N-(3-hydroxy-9,10-dioxo-9,10-dihydroanthracene-2-sulfonyl)glycine | C16 H11 N O7 S 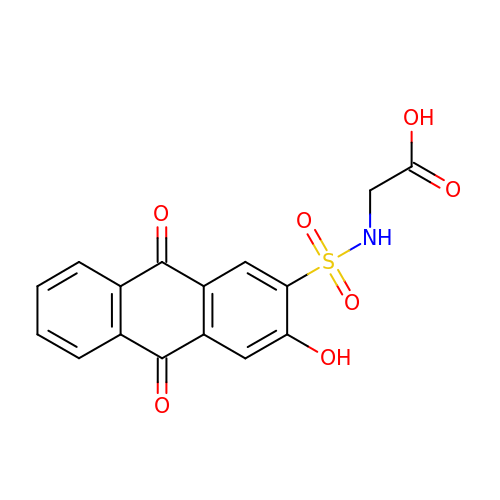| YKNJQQVUXNATBD-UHFFFAOYSA-N>MSLSIPTIKQVRAFVLRGGGADYHDQGDGHWIDDHISTPMGKYPEYRQSRRSFGINVLGTLVVEIEASDGNVGFAVTTGGEPAAYIVEKHLARFLEGARVTDIERIWDQMYNSTLYYGRKGLVINTISGVDLALWDLLGKVRREPVHQLLGGAVRDELQFYATGARPDLAQKMGFIGGKMPLHHGPSEGEEGLKKNLEELATMRERVGPDFWLMFDCWMSLDLNYATRLARGAREYGLKWIEEALPPDDYWGYAELRRNAPTGMMVTTGEHEATRWGFRMLLEMGCCDIIQPDVGWCGGVTELLKIS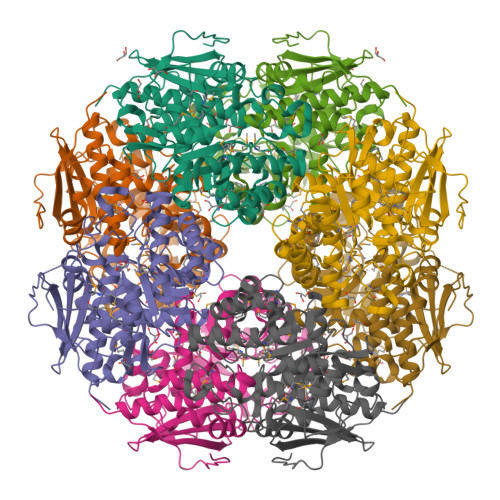ALADAHNALVVPHGSSVYSYHFVATRQNSPFAEFLMMAPKADQVVPMFHPQLLGEPVPENGRMRLSRLDQPGFGVTLNPECQLHRPYTHEGHHHHHH[8x]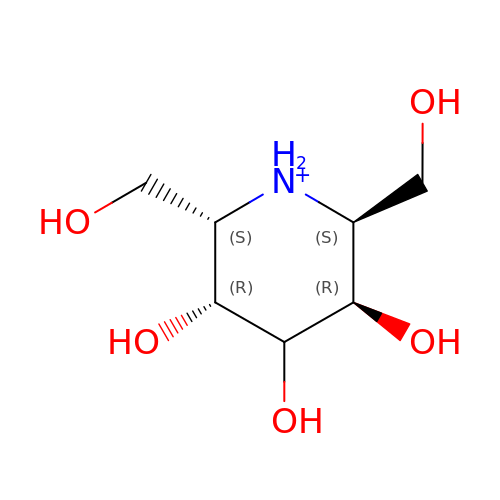(2S,3R,5R,6S)-3,4,5-TRIHYDROXY-2,6-BIS(HYDROXYMETHYL)PIPERIDINIUM | C7 H16 N O5 | CLVUFWXGNIFGNC-UNTFVMJOSA-O>MKTYNVDENGYYGEFGGAYIPEILHKCVEDLQNNYLKILESPDFQKEYDQLLRDYVGRPSPLYLAKRLSEKYGCKIYLKREDLNHTGAHAINNTIGQILLARRMGKTRIIAETGAGQHGVATATVCALMNMECIVYMGKTDVERQHVNVQKMEMLGATVVPVTSGNMTLKDATNEAIRDWCCHPSDTYYIIGSTVGPHPYPDMVARLQSVISKEIKKQLQEKEGRDYPDYLIACVGGGSNAAGTIYHYIDDERVKIVLAEAGGKGIDSGMTAATIHLGKMGIIHGSKTLVMQNEDGQIEEPYSISAGLDYPGIGPMHANLAKQKRAQVLAINDDEALNAAFELTRLEGIIPALESAHALAALEKVKFKPEDVV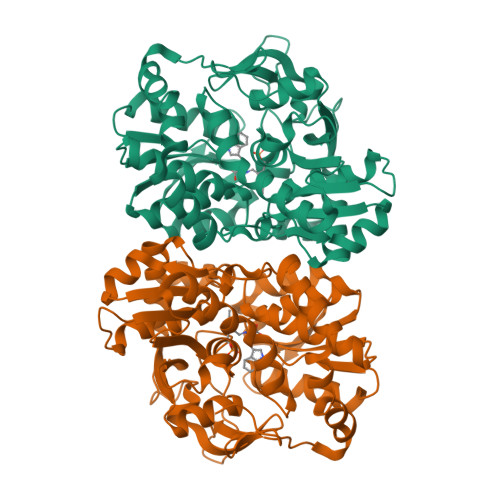VLTLSGRGDKDMETYLKYKKNSNE[4x]> GAMDKLELVNDGLNIIDFIQKNQKEIQKT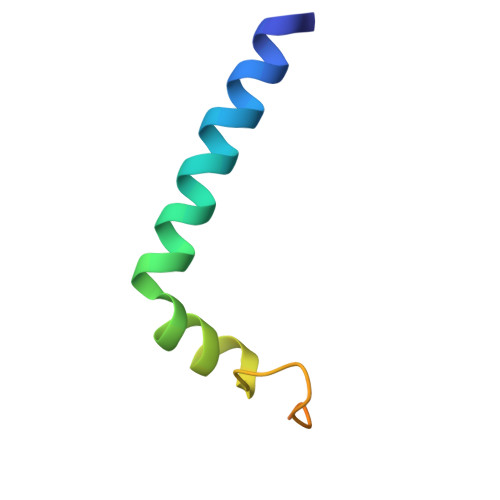YGRSSIQQPSIKDQTKAWEDFLQ> FNKIKDSVKQKIDSMGDKGTYGVSASHPLAVEEGMKVLKNGGSAVDAAIVVSYVLGVVELHASGIGGGGGMLIISKDKETFIDYRETTPYFTGNQKPHIGVPGFVAGMEYIHDNYGSLPMGELLQPAINYAEKGFKVDDSLTMRLDLAKPRIYSDKLSIFYPNGEPIETGETLIQTDLARTLKKIQKEGAKGFYEGGVARAISKTAKISLEDIKGYKVEVRKPVKGNYMGYDVYTAPPPFSGVTLLQMLKLAEKKEVYKDVDHTATYMSKMEEISRIAYQDRKKNLGDPNYVNMDPNKMVSDKYISTMKNENGDALSEAEHES;>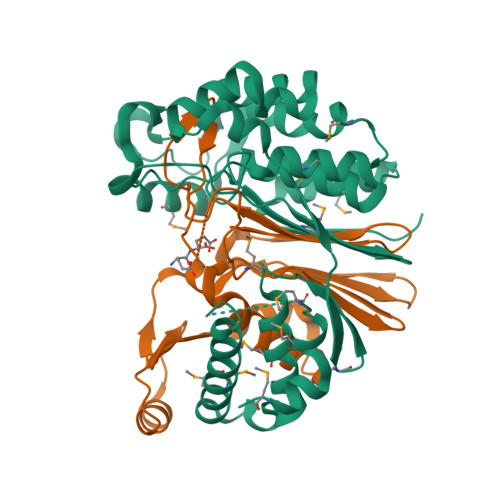 TTHFVIIDRDGTVVSSTNTLSNFFGTGKYTAGFFLNNQLQNFGSEGFNSYEPGKRSRTFMAPTVLKKDGETIGIGSPGGNRIPQILTPILDKYTHGKGSLQDIINEYRFTFEKNTAYTEIQLSSEVKNELSRKGLNVKKKVSPAFFGGVQALIKDERDNVITGAGDGRRNGTWKSNK> MKGFFAGVVAAATLAVASAGDYCGQWDWAKSTNYIVYNNLWNKNAA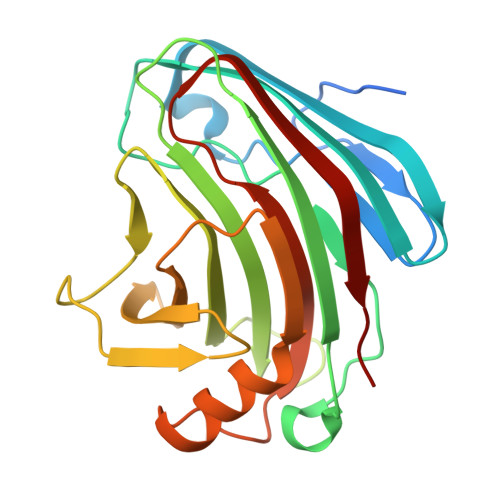ASGSQCTGVDKISGSTIAWHTSYTWTGGAATEVKSYSNAALVFSKKQIKNIKSIPTKMKYSYSHSSGTFVADVSYDLFTSSTASGSNEYEIMIWLAAYGGAGPISSTGKAIATVTIGSNSFKLYKGPNGSTTVFSFVATKTITNFSADLQKFLSYLTKNQGLPSSQYLITLEAGTEPFVGTNAKMTVSSFSAAVN> RSFRGPLLPNRPFTTVWNANTQWCLERHGVDVDVSVFDVVANPGQTFRGPDMTIFYSSQLGTYPYYTPTGEPVFGGLPQNASLIAHLARTFQDILAAIPAPDFS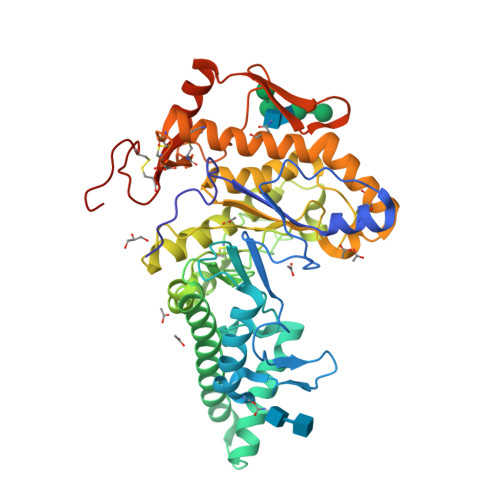GLAVIDWEAWRPRWAFNWDTKDIYRQRSRALVQAQHPDWPAPQVEAVAQDQFQGAARAWMAGTLQLGRALRPRGLWGFYGFPDCYNYDFLSPNYTGQCPSGIRAQNDQLGWLWGQSRALYPSIYMPAVLEGTGKSQMYVQHRVAEAFRVAVAAGDPNLPVLPYVQIFYDTTNHFLPLDELEHSLGESAAQGAAGVVLWVSWENTRTKESCQAIKEYMDTTLGPFILNVTSGALLCSQALCSGHGRCVRRTSHPKALLLLNPASFSIQLTPGGGPLSLRGALSLEDQAQMAVEFKCRCYPGWQAPWCERKSMWTGHHHHHH>MSPILGYWKIKGLVQPTRLLLEYLEEKYEEHLYERDEGDKWRNKKFELGLEFPNLPYYIDGDVKLTQSMAIIRYIADKHNMLGGCPKERAEISMLEGAVLDIRYGVSRIAYSKDFETLKVDFLSKLPEMLKMFEDRLCHKTYLNGDHVTHPDFMLYDALDVVLYMDP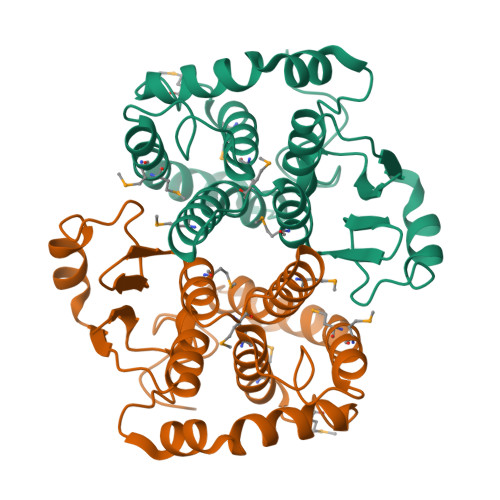MCLDAFPKLVCFKKRIEAIPQIDKYLKSSKYIAWPLQGWQATFGGGDHPPKSDGSSMGSSHHHHHHSSGLVPR[2x]4'-(6,7-dimethoxyindeno[1,2-c]pyrazol-3-yl)biphenyl-4-ol | 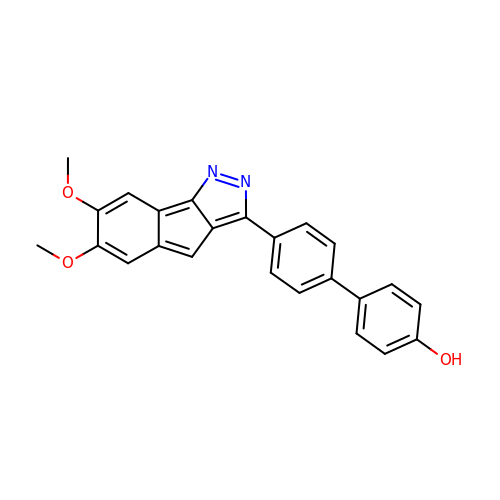C24 H18 N2 O3 | XYLHIQKMKPVWAM-UHFFFAOYSA-N(2R,3S,4R,5R)-5-(HYDROXYMETHYL)PIPERIDINE-2,3,4-TRIOL | C6 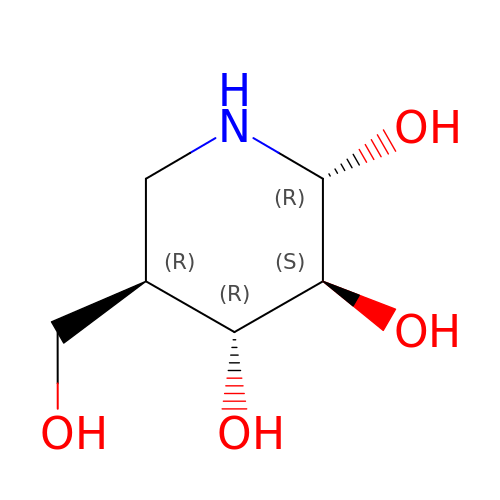H13 N O4 | BHOYFRIRWXBNHP-ARQDHWQXSA-N Here, we identify an alternative approach to sulfoquinovoside hydrolysis that is adopted by these organisms and discover a family of SQases belonging to a new glycoside hydrolase family (GH188). These new SQases operate through an oxidoreductive mechanism that results in net hydrolysis and involves a catalytic NAD+ cofactor. The SqgA proteins adopt a two-domain fold with an N-terminal dinucleotide binding Rossmann domain and a C-terminal α/β dimerization domain. The structures reveal homodimers, consistent with molar mass analysis using size-exclusion chromatography-multiangle laser light scattering in solution.

Two other orthologues, ArSqgA from Arthrobacter sp. U41 and CrSqgA from Cryobacterium sp. TMT2–4, also cleaved α-PNPSQ. To gain insight into the molecular basis of catalysis, we determined the 3D structures of FlSqgA and ArSqgA using X-ray crystallography. Crystals of FlSqgA and ArSqgA were grown in the presence of NAD+ (or a ternary complex of ArSqgA with citrate and NAD+) and diffracted to 2.35 and 2.65 (or 1.95) Å, respectively. Clear, contiguous density was seen in both structures within a cleft between the two domains that allowed modeling of a single molecule of NAD+ bound in an extended conformation in each monomer with its nicotinamide ring projecting into a polar pocket. Superposition of ArSqgA·NAD+ binary and ArSqgA·NAD+·SQ ternary complexes (backbone RMSD of 0.5 Å over 364 residues) revealed no major structural changes upon binding SQ. The active site was also largely unchanged with the notable exception of the Tyr136 residue in some of the individual protomer chains, which rotated 72° about the Cα–Cβ bond to engage with C2–OH of SQ in the ArSqgA·NAD+·SQ complex.

>[2x]MGSSHHHHHHSSGMSLPTAEAVRTIRYGLIGAGHMAREHVRNLALIPGSLITAVSDPQPSSLEETVAEIGYEVTTFPDHRELLVSGLVDALVIASPNDTHLDILKDIFSNQMKLPVLVEKPVCTTAAQADELESLAAGYSAPVWVAMEYRYMPPVQELIQAAHGGKLGNVFMLSIVEHRFPFLHKVDAWNRFNERTGGTLVEKCCHFFDLMRLILQDEPTRIYASGGHDVNHMDELYEGRVSDMIDNAYVVVDFKSGRRAMLELSMFAEGSKFQERISIVGDAAKIECLIPVAASHWIEGDESEAVVEFSPRSPLGPETHEVPVDEAVLAAGAHHGSTYYEHLGYRKAILGEGPVEVTVADGLQSVRMGLAAERSIIEGRPVELLSANSAVS> GSPEFMENLVTLSRQGIENLMKLENRKEPWIVVLYAPWCPFCQAMEASYDELADKLAGSGIKVAKFRADGDQKEFAKQELQLGSFPTILVFPKNSSRPIKYPSEKRDVESLTSFLLEHHHHHH

The first step is the reaction between the key enzyme APS reductase (APR) and APS to generate a thiosulfonate-enzyme intermediate. In contrast to the cooperation of a sulfonucleotide reductase and a thioredoxin in prokaryote systems, in plants, the protein involved in the pathway is only a single polypeptide which consists of two distinct domains: a sulfonucleotide reductase-like one and a thioredoxin-like one. In plants, the C-terminal domain of APR itself serves the function like thioredoxin. To gain more insights into the C-terminal redox domain of plant-type APR, here we present a comprehensive structural and biochemical study of Arabidopsis thaliana APR1 (AtAPR1).

To provide insights into the structural basis of the AtAPR1 redox domain, we produced and crystallized the C-terminal redox domain of Arabidopsis APR1 (residues 353–461) and obtained crystal belonging to the tetragonal space group with the following unit-cell dimensions: a = b = 58.2, c = 86.7 Å. Finally, the crystal structure of the AtAPR1 redox domain was refined to Rwork = 17.9% and Rfree = 25.0% with high-quality backbone geometry checked by Ramachandran plot. The structure of the AtAPR1 redox domain is a compact spherical molecule comprising a central core of five-stranded β-sheets flanked on either side by four helices. The fold of the redox domain arranged in the order β1-α1-β2-α2-β3-α3-β4-β5-α4 is similar to the thioredoxin fold but not glutaredoxin fold. The redox-active motif (Cys33-Pro34-Phe35-Cys36) is located at the N-terminal end of the α2-helix, consisting of residues Pro34 to Leu50. The packing of the sandwich-like architecture is mainly maintained by hydrophobic interactions between the sheet and helices. Surface potential distribution of the redox domain shows most positive-charged residues around the redox-active motif. The molecular mass of the AtAPR1 redox domain in solution determined by size-exclusion chromatography was about 13 kDa, which indicates the monomeric form of the AtAPR1 redox domain. As a whole, the structural information indicates that the C-terminal redox domain of plant-type APR1 adopts a non-canonical thioredoxin fold with exceptional orientations of helices α2, α3, and α4, which is quite different from typical thioredoxins. Notably, the surface charge distribution around the GSH binding site of the AtAPR1 redox domain is ideally complementary to the charge of GSH, but other thioredoxins are not.> MTVFRQENVDDYYDTGEELGSGKFAVVKKCREKSTGLQYAAKFIKKRRTKSSRRGVSREDIEREVSILKEIQHPNVITLHEVYENKTDVILILELVAGGELFDFLAEKESLTEEEATEFLKQILNGVYYLHSLQIAHFDLKPENIMLLDRNVPKPRIKIIDF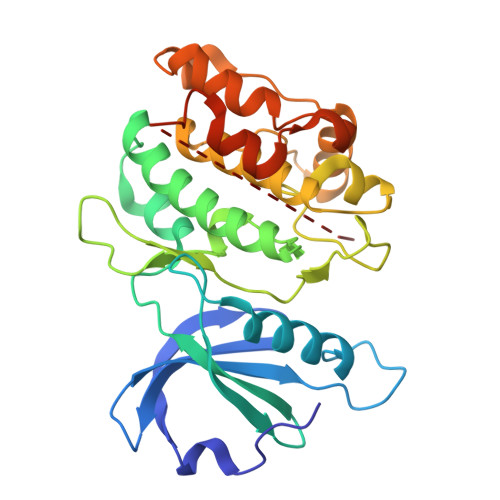GLAHKIDFGNEFKNIFGTPEFVAPEIVNYEPLGLEADMWSIGVITYILLSGASPFLGDTKQETLANVSAVNYEFEDEYFSNTSALAKDFIRRLLVKDPKKRMTIQDSLQHPWIKPKDTQQALSSAWSHPQFEK>GPAMKKLKPAPFYFQPFSKKQLKVLTWWRKASPVSDKDGIICDGSIRAGKTIVMSFSYVMWAMDTFNEQNFGMAGKTIGALRRNVITPLKRMLKSRGYRVKDHRADNYLTITFKGKTNYFYLFGGKDESSQDLIQGITLAGMFFDEVALMPESFVNQATARCSVDGAKLWFNCNPAGPYHWFKVEYLDKLDEKNLLHLHFTMDDNLSLSKQVKERYQRMYKGVFYQRYILGLWVLAEGIIYDMFDQDEHVVPTVPRPYEKYYVSCDYGTQNPTTFGLWGLYNGVWYKVKEYHYDGRKENKQKTDQEYYEDLMKFIEDIEKHKFKGVIVDPSAASFIALLRQKGIKVIKAKNDVLDGIRNVATALNKKMILYNDCCKETFREYSSYVWDEKAAERGEDKPVKQNDHQLDADRYFVNTILFGNKLRAVPSLY[3x]

Most dsDNA bacteriophages and viruses utilize a powerful DNA translocation motor to package their unit-length genome into a preformed procapsid. A central component of the motor, large terminase, consists of an N-terminal adenosine triphosphatase (ATPase) domain comprising ASCE (Additional Strand Catalytic glutamate) and lid subdomains, and a C-terminal nuclease domain, connected by a short linker sequence. While both domains are involved in interaction with DNA DNA translocation is powered by the ASCE subdomain using energy released coinciding with ATP hydrolysis. The nuclease domain is responsible for cleavage of the genomic DNA concatemer at both the initiation and completion stages of viral DNA packaging.

Subsequent soaking of these crystals in cryo-protectant containing a high concentration of NaCl resulted in a transition from R32 to C2 crystal form (Crystal form 2) with each of the ATPase domains of the three subunits related by the crystallographic 3-fold axis adopting a unique stable position. The final α-helix (α6) of the nuclease domain is followed by an ordered extended C-terminal loop or ‘arm’ proximal to the ATPase active site that contains a bound sulphate ion, which was present in the crystallization condition. Initial attempts to produce diffracting crystals of ligand-bound complexes of the full-length protein failed, despite thermofluor data showing stabilization of the protein in the presence of magnesium ions and either ATP-γ-S or ADP (ΔTm of 7.8 and 2.3 respectively), Inspection of the structure containing bound sulphate ion in the ATPase active site showed that in crystal form 2, the C-terminal arm of the nuclease domain occludes the ATPase active site and likely requires significant reorganization to accommodate an ATP analogue. The C-terminal arm, residues 418–427 of the nuclease domain, lies close to the ATPase active site and thus may play a role in ATP binding and/or hydrolysis. Indeed, closer analysis reveals that this ordered extended turn contributes to the active site through an arginine residue (R421) at the tip of the C-terminal arm, that is in proximity to the sulphate ion bound in the active site. Additionally, the carbonyl oxygen of the preceding residue, L420, formed a hydrogen bonding interaction with R44 of the P-loop of the lid subdomain. Superposition of the structures for the full-length protein and the truncated protein (with bound sulphate or ATP-γ-S, respectively) positions R421 close to the α-phosphate of the ATP-γ-S. ATP bound in the monomer active site cannot be hydrolyzed without the participation of the trans- arginine finger from an adjacent subunit in the assembled pentamer, which requires significant rotation of the nuclease domain with respect to the ATPase domain. This monomer conformation is stabilized, or ‘locked’, by the C-terminal arm.Based on the structure-function knowledge of the RNase A superfamily we have engineered a chimera that combines RNase 1 highest catalytic activity with RNase 3 unique antipathogen properties. Based on the RNase 1 scaffold we incorporated specific regions essential for RNase 3 unique anti-pathogen activities within the RNase A superfamily. The solved crystal structures confirmed that all the chimera proteins reproduce the kidney-shaped folding typical of the RNase A superfamily and thus keep the fold of the templates used in their design, as suggested by circular dichroism and molecular dynamics analysis. Nonetheless, the structures that incorporated the key features related to RNase 3 antimicrobial activity retained the overall RNase 1 active site conformation together with the essential structural elements for binding to the human ribonuclease inhibitor (RNHI), ensuring non-cytotoxicity.

Next, a second variant (RNase 3/1-v2) was designed to incorporate loop L7, a region characteristic of RNase 3 and shared with other antimicrobial RNases, but absent in RNase 1. Two crystal structures of RNase 3/1-v2 were solved, one free and the other in complex with phosphate ions. No significant differences at the structural level were observed, with an RMSD of 0.4 Å. In both cases the model is traced till residue Ala134, being shorter than its full sequence because no electron density is observed for the C-terminal end. As observed in RNase 3/1-v1, the residues Phe132 and Ser134 in -v2 variant have a different position than their RNase 1 counterparts, altering the B1 site cavity conformation. Interestingly, the R1-L1 (D17-R27) was hard to build in both crystal structures of RNase 3/1-v2 due to poor electron density map, in opposition to the equivalent L1 loop in RNase 3/1-v1. A close inspection of phosphate anions in RNase 3/1-v2 indicates that one phosphate anion is interacting with the catalytic triad. The other phosphates are bound at the protein surface, where PO4 anions n° 1 and 2 might correspond to alternative positions of the same binding site. Comparison of free and phosphate bound RNase 3/1-v2 structures highlights Arg 101 residue, which gets fixed at only one position upon phosphate interaction. Presence of a phosphate anion interacting with the enzyme catalytic triad confirms the conservation of the active site groove in both -v2 and -v3 structures.

> MRPPQFTRAQWFAIQHIDSDSSPSSSSRYCTIAMRAINNYRWRCKPVNTFVHEPLVDVQNVCFQEKVTCKNGQGNCYRSRFRMHITDCRLTNGSRYPNCRYRTRPGRRHIIVACENRDPRDSPRYPYVPVHFDASV>LQLTESDIMPFNFDQRIDRRHSDSLKWKKYADRDILPLWIADTDFRAADCIIDALQQRVQQGVFGYGVTSEALAEVAIERMESRFGWKIQPEWLVFLPGVVTGINIAVRAFTEAHQSTVSATPIYPPFFLAPKLAGRQHLSAALRLEQQRWVLDLDSHEDRMSGNEKLLLLCNPHNPGGTVYRRKELEAQLRFAQRHDLLVCSDEIHCDLVLEPGVQHIPFASLSDDAAQRSITLMSPSKSFNIAGLGASLAVIPNPELRARFNRMRKGMVPDVDVLAYVAASAAWREGQPWLDAQLDYLRANRDMLAQHVNRLPGLSMVTPEASFLGWIDASGLGVADPALFFEKHGLGFSSGRDFGNDRFVRFNFGCPRQ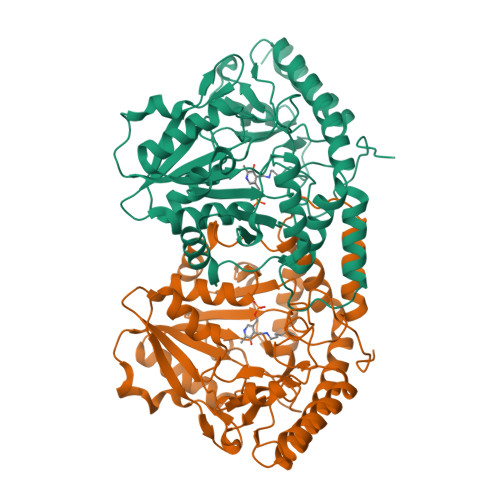LLEEALQRMTRALTSGY[12x]>[6x]SEISRQEFQRRRQALVEQMQPGSAALIFAAPEVTRSADSEYPYRQNSDFWYFTGFNEPEAVLVLIKSDDTHNHSVLFNRVRDLTAEIWFGRRLGQDAAPEKLGVDRALAFSEINQQLYQLLNGLDVVYHAQGEYAYADVIVNSALEKLRKGS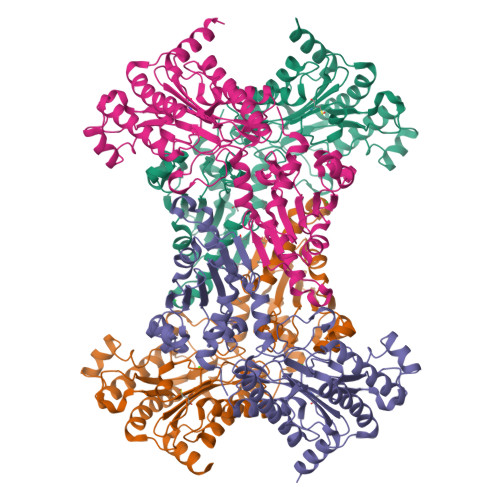RQNLTAPATMIDWRPVVHEMRLFKSPEEIAVLRRAGEITAMAHTRAMEKCRPGMFEYHLEGEIHHEFNRHGARYPSYNTIVGSGENGCILHYTENECEMRDGDLVLIDAGCEYKGYAGDITRTFPVNGKFTQAQREIYDIVLESLETSLRLYRPGTSILEVTGEVVRIMVSGLVKLGILKGDVDELIAQNAHRPFFMHGLSHWLGLDVHDVGVYGQDRSRILEPGMVLTVEPGLYIAPDAEVPEQYRGIGIRIEDDIVITETGNENLTASVVKKPEEIEALMVAARKQ>[2x]GAMGMKKIEVDLVRTKVYNLLKEMILNHELKLGEKLNVRELSEKLGISFTPVRDALLQLATEGLVKVVPRVGFFVT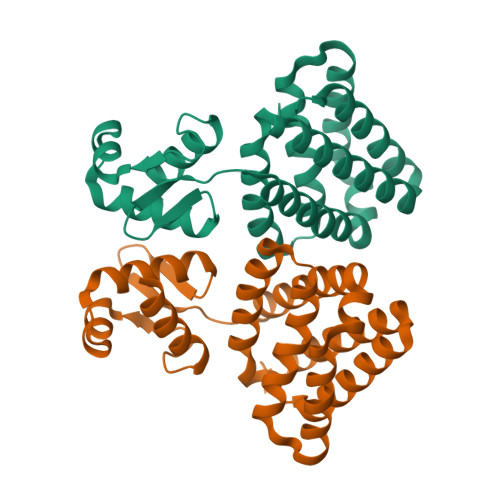DVDEKFIRETIETRIMMEVFCLENYFDKIAGSEELLEIKGEIDDVEKSAKREIFDDSDERLHKLFIRASGNELIISLYEKIWDRIDLVRHLNERYVVSNREHKELIERIISGDKEGAIEKLKEHLKNVEAETIKNLYTYERS> MNNLHRELAPISEAAWKQIDDEARDTFSLRAAGRRVVDVPEPAGPTLGSVSLGHLETGSQTDGVQTSVYRVQPLVQVRVPFTVSRADIDDVERGAVDLTWDPVDDAVAKLVDTEDTAILHGWEEAGITGLSEASVHQPVQMPAELEQIDDAVSGACNVLRLADVEGPYDLVLPQQLYTQVSETTDHG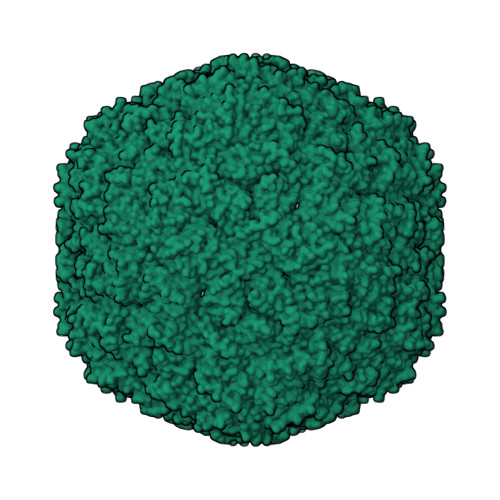VPVVDHLTQLLSGGEVLWAPAARCALVVSRRGGDSCLFLGRDVSIGYLSHDAQTVTLYLEESFTFRVHQPDAAVALV> SMSSFEGQMAEYPTISIDRFDRENLRARAYFLSHCDKDHMKGLRAPTLKRRLECSLKVYLYCSPVTKELLLTSPKYRFWKKRIISIEIETPTQISLVDEASGEKEEIVVTLLPAGHCPGSVMFLFQGNNGTVLYTGDFRLAQGEAARMELLHSGGRVKDIQSVYLDTTFCDPRFYQIPSREECLSGVLELVRSWITRSPYHVVWLNCKAAYGYEYLFTNLSEELGVQVHVNKLDMFRNMPEILHHLTTDRNTQIHACRHPKAEEYFQWSKLPCGITSRNRIPLHIISIKPSTMWFGERSRKTNVIVRTGESSYRACFSFHSSYSEIKDFLSYLCPVNAYPNVIPVGTTMDKVVEILKPLCRS

Artemis (SNM1C/DCLRE1C) is an endonuclease that plays a key role in development of B- and T-lymphocytes and in dsDNA break repair by non-homologous end-joining (NHEJ). Artemis is phosphorylated by DNA-PKcs and acts to open DNA hairpin intermediates generated during V(D)J and class-switch recombination. Artemis belongs to a superfamily of nucleases containing metallo-β-lactamase (MBL) and β-CASP (CPSF-Artemis-SNM1-Pso2) domains. The overall fold of the catalytic core of Artemis is similar to that of SNM1A and SNM1B (2 Å backbone RMSD); it has all the key structural characteristics of human MBL fold nucleases, with the di-metal containing active site at the interface between the MBL and β-CASP domains.

We solved structures of three Artemis variants D37A, H33A and an Omenn syndrome patient mutation, H35D. We crystallized three forms of truncated Artemis (aa 1–361) with substitutions in several of these metal ion co-ordinating residues, i.e. D37A, H33A, and the Omenn Syndrome patient mutation H35D. The overall architecture of the three variants is almost identical to WT Artemis. The D37A structure crystallizes with only one nickel ion (M1); Both the H33A and H35D variants exhibited loss of the M1 ion. By contrast, all three variants retained the Zn ion in the zinc finger-like motif of the β-CASP domain. Histidines 33 and 35 are the first two histidine residues in the HxHxDH motif (M1 binding) in the active site. In the absence of active site metal ions, the loop comprising residues 113–119 moves away from the active site and a small rearrangement occurs in α8 (residues 348–358). In both the H33A and H35D variants, α8 moves slightly closer towards β14, compared to the WT and D37A variant. In H33A and H35D variants, both β-strand E and α-helix E shifted upward and away from the zinc finger like motif. Differential scanning fluorimetry (DSF) analyses showed that both H33A and H35D variants are substantially destabilized with ΔTm around -13°C compared to WT Artemis. Our D37A, H33A, and H35D variants lost the ability to digest DNA substrate in vitro, in accord with results with full-length variants.>GGDQRFGDLVFRQLAPNVWQHTSYLDMPGFGAVASNGLIVRDGGRVLVVDTAWTDDQTAQILNWIKQEINLPVALAVVTHAHQDKMGGMDALHAAGIATYANALSNQLAPQEGLVAAQHSLTFAANGWVEPATAPNFGPLKVFYPGPGHTSDNITVGIDGTDIAFGGCLIKDSKAKSLGNLGDADTEHYAASARAFGAAFPKASMIVMSHSAPDSRAAITHTARMADKLR[2x]

The bacterial metallo-β-lactamases (MBLs) catalyze the inactivation of β-lactam antibiotics. Class B members, known as the metallo-β-lactamases (MBLs), are structurally distinct from the Class A, C, and D enzymes, require one or two zinc ions for catalytic activity, and are not inhibited by currently approved therapeutics. One variant of significance is NDM-4, first identified in 2012 (17). Although it differs from NDM-1 by a single amino acid substitution, namely M154L, it demonstrates increased enzymatic activity against the carbapenems and several cephalosporins.

The crystals of the NDM-4/l-captopril complex utilized for this analysis were also grown from poly(ethylene glycol) 3350 and belonged to the P21 space group. This time, however, there were two monomers in the asymmetric unit. The model of the NDM-4/l-captopril complex was refined to an overall R-factor of 20% at 1.3 Å resolution. The reverse turn in the apoenzyme structure that adopts two distinct conformations (Ala 55 to Val 58) is a distorted Type I turn in the NDM-4/l-captopril model. In both subunits of the NDM-4/l-captopril model, the region delineated by Leu 65 to Ala 72 adopts two distinct conformations, labeled A and B as shown in Figure 3A. In conformation B, Cζ of Phe 70 lies within 3.6 Å of a carboxylate oxygen of the l-captopril ligand. The sulfur of the ligand lies within 2.2. Å and 2.1 Å of Zn1 and Zn2, respectively. The bridging solvent in the apoenzyme model, as well as three additional waters are extruded from the vicinity of the binuclear metal center upon l-captopril binding. As a consequence, the coordination geometry surrounding Zn2 changes from octahedral to distorted tetrahedral shown in Figure 3C. In addition to its interaction with the binuclear metal center, the ligand also lies within hydrogen bonding distance to an ordered water molecule and the backbone amide nitrogen of Asn 220. The determined Ki for l-captopril was 164 μM and 210 μM with a corresponding LE of 0.37 and 0.36 against NDM-1 and NDM-4, respectively.> SNAMSAIPITPTKRIRRNLFDDAPATPPRPLKRKKLQFTDVTPESSPEKLQFGSQSIFLRTKALLQKSSELVNLNSSDGALPARTAEYEQVMNFLAKAISEHRSDSLYITGPPGTGKTAQLDMIIRQKFQSLPLSLSTPRSKDVLRHTNPNLQNLSWFELPDGRLESVAVTSINCISLGEPSSIFQKIFDSFQDLNGPTLQIKNMQHLQKFLEPYHKKTTFVVVLDEMDRLLHANTSETQSVRTILELFLLAKLPTVSFVLIGMANSLDMKDRFLSRLNLDRGLLPQTIVFQPYTAEQMYEIVIQKMSSLPTIIFQPMAIKFAAKKCAGNT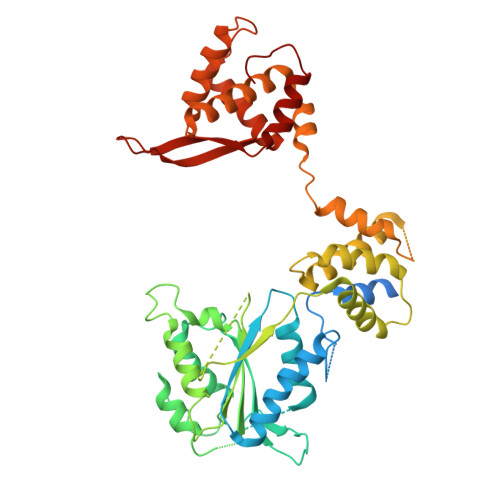GDLRKLFDVLRGSIEIYELEKRFLLSPTRGSLNSAQVPLTPTTSPVKKSYPEPQGKIGLNYIAKVFSKFVNNNSTRTRIAKLNIQQKLILCTIIQSLKLNSDATIDESFDHYIKAITKTDTLAPLQRNEFLEICTILETCGLVSIKKTKCKGKTKRFVDKIDVDLDMREFYDEMTKISILKPFLH> LGLRRAGVRKALHDPFEDGALVLYEPPAISAHDLIKADKEKLPVHVVVDPVLSKVLRPHQREGVKFLWDCVTGRRIENSYGCIMADEMGLGKTLQCITLIWTLLKQSPDCKPEIDKVIVVSPSSLVRNWYNEVGKWLGGRVQPVAIDGGSKDEIDSKLVNFISQQGMRIPTPILIISYETFRLHAEVLHKGKVGLVICDEGHRLKNSDNQTYLALNSMNAQRRVLISGTPIQNDLLEYFSLVHFVNSGILGTAQEFKKRFEIPILKGRDADASDKDRAAGEQKLQELISIVNRCLIRRTSDILSKYLPVKIEQVVCCNLTPLQKELYKLFLKQAKPVE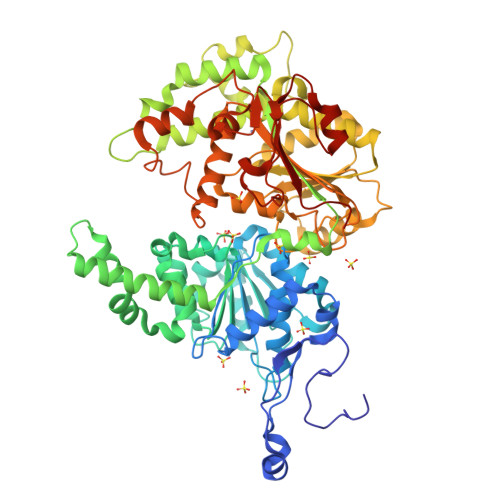SLQTGKISVSSLSSITSLKKLCNHPALIYEKCLTGEEGFDGALDLFPQNYSTKAVEPQLSGKMLVLDYILAMTRTTTSDKVVLVSNYTQTLDLFEKLCRNRRYLYVRLDGTMSIKKRAKIVERFNNPSSPEFIFMLSSKAGGCGLNLIGANRLVMFDPDWNPANDEQAMARVWRDGQKKTCYIYRLLSTGTIEEKILQRQAHKKALSSCVVDEEQDVERHFSLGELRELFSLNEKTLSDTHDRFRCRRCVNGRQVRPPPDDSDCTCDLSNWHHCADKRGLRDPVLQASWDAAVSFVFHQRSHEDQR> MDLEMMLDEDYKEGICLIDFSQIALSTALVNFPDKEKINLSMVRHLILNSIKFNVKKAKTLGYTKIVLCIDNAKSGYWRRDFAYYYKKNRGKAREESTWDWEGYFESSHKVIDELKAYMPYIVMDIDKYEANDHIAVLVKKFSLEGHKILIISSDGDFTQLHKYPNVKQWSPMHKKWVKIKSGSAEIDCMTKILKGDKKDNVASVKVRSDFWFTRVEGERTPSMKTSIVEAIANDRE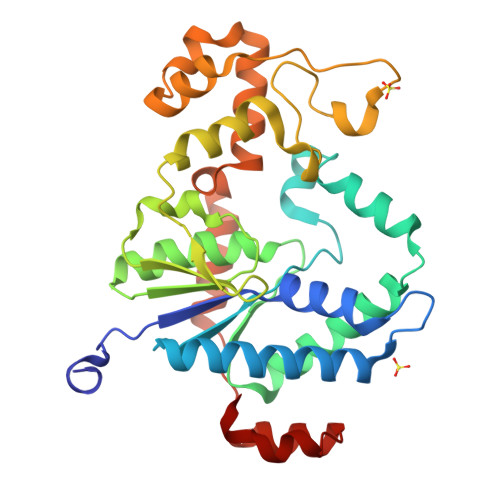QAKVLLTESEYNRYKENLVLIDFDYIPDNIASNIVNYYNSYKLPPRGKIYSYFVKAGLSKLTNSINEF5-{3-methoxy-4-[(4-methoxybenzyl)oxy]benzyl}pyrimidine-2,4-diamine | C20 H22 N4 O3 | 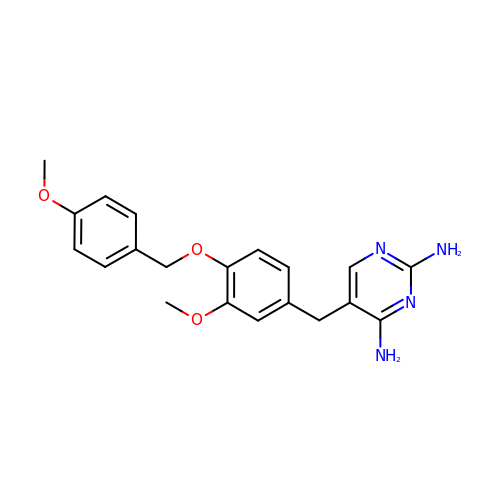MYQAUKPBNJWPIE-UHFFFAOYSA-N~{N}-[[3,4-bis(fluoranyl)phenyl]methyl]-4-[(4-methylpiperazin-1-yl)methyl]aniline | C19 H23 F2 N3 | 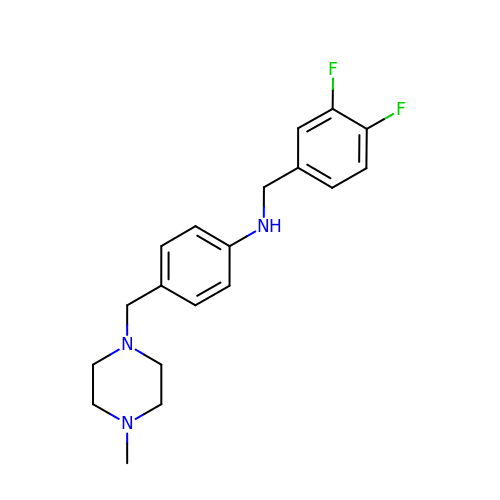HJMKUKHAURUGEC-UHFFFAOYSA-N>[2x]SMADLSSKRSRVVGVVVPLIHTNFADEIIKGLYETTISSGYELLITYLDEDEDHQYQVFQTLLSRQVGAVFMLSLDIPSWMIDKLLEEQISVISLTALLSEQISAVTSNEFEMMNSIVDYLIDMGHKNIALVGDTKLTTNISSTRRTNFIKSMTDHNLAYENIFLYGNDHSYETGYTSVTTGYDINQLPFTAAIATADMVGQGLINAMSDHGKTVPEDLSIVTIDGLQQTEIARPKLTTVKQDFPEI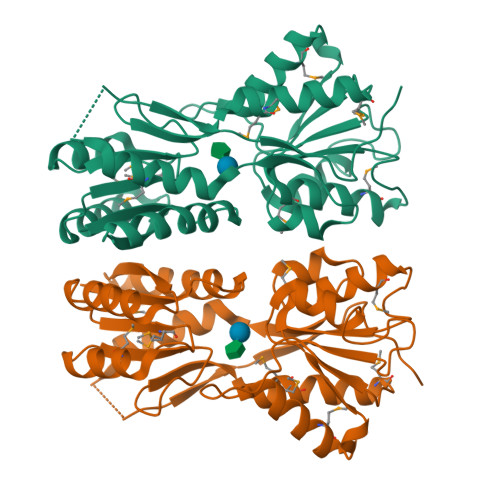GRIAMQLFLDSDSEKTEPQIIYIPTELIQRDSVLNLNSTK>THPIIHDLENRYTSKKYDPSKKVSQEDLAVLLEALRLSASSINSQPWKFIVIESDAAKQRMHDSFANMHQFNQPHIKACSHVILFANKLSYTRDDYDVVLSKAVADKRITEEQKEAAFASFKFVELNCDENGEHK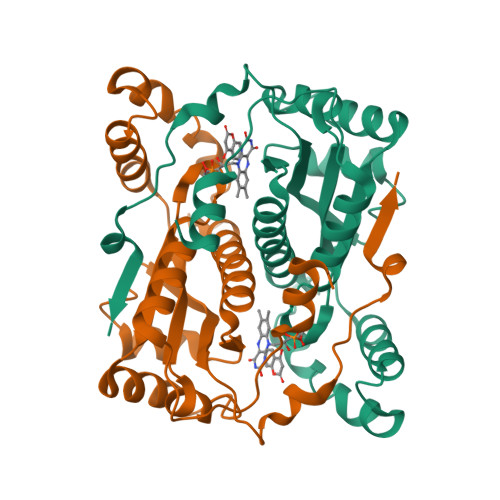AWTKPQAYLALGNALHTLARLNIDSTTMEGIDPELLSEIFADELKGYECHVALAIGYHHPSEDYNASLPKSRKAFEDVITIL[2x]> MLKRKQSSRVEAQPVTDFGPDESLSDNADILWINKPWVHSLLRI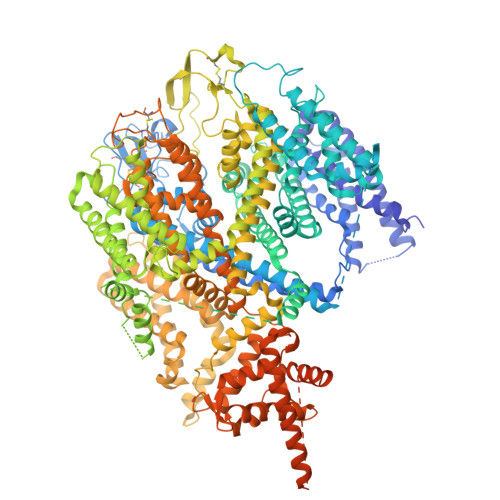CAIISVISVCMNTPMTFEHYPPLQYVTFTLDTLLMFLYTAEMIAKMHIRGIVKGDSSYVKDRWCVFDGFMVFCLWVSLVLQVFEIADIVDQMSPWGMLRIPRPLIMIRAFRIYFRFELPRTRITNILKRSGEQIWSVSIFLLFFLLLYGILGVQMFGTFTYHCVVNDTKPGNVTWNSLAIPDTHCSPELEEGYQCPPGFKCMDLEDLGLSRQELGYSGFNEIGTSIFTVYEAASQEGWVFLMYRAIDSFPRWRSYFYFITLIFFLAWLVKNVFIAVIIETFAEIRVQFQQMWGSRSSTTSTATTQMFHEDAAGGWQLVAVDVNKPQGRAPACLQKMMRSSVFHMFILSMVTVDVIVAASNYYKGENFRRQYDEFYLAEVAFTVLFDLEALLKIWCLGFTGYISSSLHKFELLLVIGTTLHVYPDLYHSQFTYFQVLRVVRLIKISPALEDFVYKIFGPGKKLGSLVVFTASLLIVMSAISLQMFCFVEELDRFTTFPRAFMSMFQILTQEGWVDVMDQTLNAVGHMWAPVVAIYFILYHLFATLILLSLFVAVILDNLELDEDLKKLKQLKQSEANADTKEKLPLRLRIFEKFPNRPQMVKISKLPSDFTVPKIRESFMKQFIDRQQQDTCCLLRSLPTTSSSSCDHSKRSAIEDNKYIDQKLRKSVFSIRARNLLEKETAVTKILRACTRQRMLSGSFEGQPAKERSILSVQHHIRQERRSLRHGSNSQRISRGKSLETLTQDHSNTVRYRNAQREDSEIKMIQEKKEQAEMKRKVQEEELRENHPYFDKPLFIVGREHRFRNFCRVVVRARFNASKTDPVTGAVKNTKYHQLYDLLGLVTYLDWVMIIVTICSCISMMFESPFRRVMHAPTLQIAEYVFVIFMSIELNLKIMADGLFFTPTAVIRDFGGVMDIFIYLVSLIFLCWMPQNVPAESGAQLLMVLRCLRPLRIFKLVPQMRKVVRELFSGFKEIFLVSILLLTLMLVFASFGVQLFAGKLAKCNDPNIIRREDCNGIFRINVSVSKNLNLKLRPGEKKPGFWVPRVWANPRNFNFDNVGNAMLALFEVLSLKGWVEVRDVIIHRVGPIHGIYIHVFVFLGCMIGLTLFVGVVIANFNENKGTALLTVDQRRWEDLKSRLKIAQPLHLPPRPDNDGFRAKMYDITQHPFFKRTIALLVLAQSVLLSVKWDVEDPVTVPLATMSVVFTFIFVLEVTMKIIAMSPAGFWQSRRNRYDLLVTSLGVVWVVLHFALLNAYTYMMGACVIVFRFFSICGKHVTLKMLLLTVVVSMYKSFFIIVGMFLLLLCYAFAGVVLFGTVKYGENINRHANFSSAGKAITVLFRIVTGEDWNKIMHDCMVQPPFCTPDEFTYWATDCGNYAGALMYFCSFYVIIAYIMLNLLVAIIVENFSLFYSTEEDQLLSYNDLRHFQIIWNMVDDKREGVIPTFRVKFLLRLLRGRLEVDLDKDKLLFKHMCYEMERLHNGGDVTFHDVLSMLSYRSVDIRKSLQLEELLAREQLEYTIEEEVAKQTIRMWLKKCLKRIRAKQQQSCSIIHSLRESQQQELSRFLNPPSIETTQPSEDTNANSQDNSMQPETSSQQQLLSPTLSDRGGSRQDAADAGKPQRKFGQWRLPSAPKPISHSVSSVNLRFGGRTTMKSVVCKMNPMTDAASCGSEVKKWWTRQLTVESDESGDDLLDILEDEVDAGSDYKDDDDKGSDYKDDDDK> CPSVCRCDRNFVYCNERSLTSVPLGIPEGVTVLYLHNNQINNAGFPAELHNVQSVHTVYLYGNQLDEFPMNLPKNVRVLHLQENNIQTISRAALAQL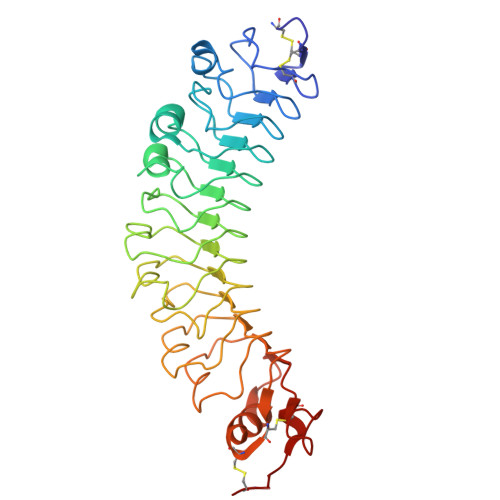LKLEELHLDDNSISTVGVEDGAFREAISLKLLFLSKNHLSSVPVGLPVDLQELRVDENRIAVISDMAFQNLTSLERLIVDGNLLTNKGIAEGTFSHLTKLKEFSIVRNSLSHPPPDLPGTHLIRLYLQDNQINHIPLTAFANLRKLERLDISNNQLRMLTQGVFDHLSNLKQLTARNNPWFCDCSIKWVTEWLKYIPSSLNVRGFMCQGPEQVRGMAVRALNMNLLSCP>MTSLFDAPTLQRVTVFTGSALGSSSLYTQAAQTLAKTAVDRGIDLVYGGGKVGLMGIVADAFLESGGEAFGVITESLMKGELGHEKLTELEIVPDMHIRKRRMAELGDGFIAMPGGAGTLEELFEVWTWQQLGIHQKPV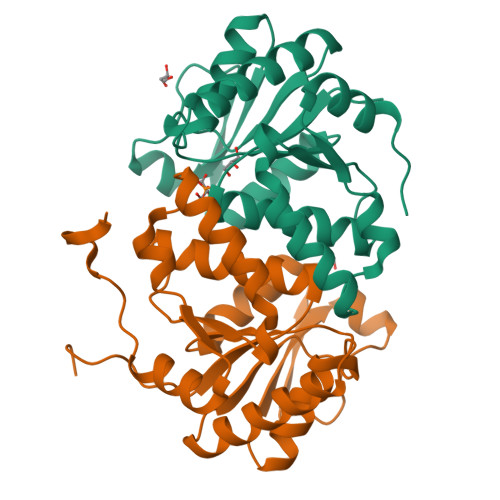ALYDVDGFWQPLLEMLEQMTQRGFIKRDFFECLIVESDPHALLKAMQTWTPPAPKWLEHHHHHH[4x]> ESQPDPMPDDLHKSSEFTGTMGNMKYLYDDHYVSATKVKSVDKFLAHDLIYNISDKKLKNYDKVKTELLNEDLAKKYKDEVVDVYGSNYYVNCYFSSKDNKWWPGKTCMYGGITKHEGNHFDNGNLQNVLVRVYENKRNTISFEVQTDKKSVTAQELDIKARNFLINKKNLYEFNSSPYETGYIKFIENNGNTFWYDMMPAPGDKFDQSKYLMMYNDNKTV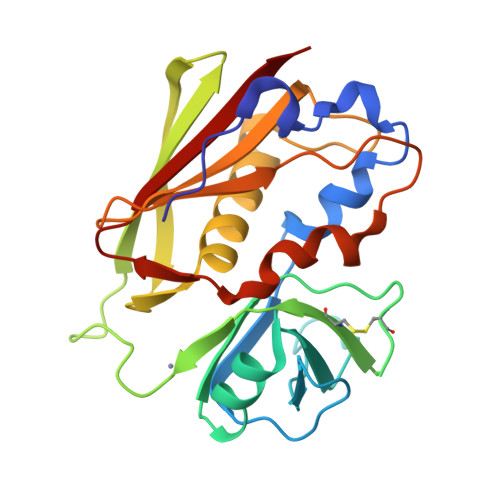DSKSVKIEVHLTTKNG>RTFLNLTKPLCEVNSWHILSKDNAIRIGEDAHILVTREPYLSCDPQGCRMFALSQGTTLRGRHANGTIHDRSPFRALISWEMGQAPSPYNTRVECIGWSSTSCHDGMSRMSICMSGPNNNASAVVWYGGRPITEIPSWAGNILRTQESECVCHKGVCPVVMTDGPANNRAATKIIYFKEGKIQKIEELAGNAQHIEECSCYGAGGVIKCICRDNWKGANRPVITIDPEMMTHTSKYLCSKVLTDTSRPNDPTNGNCDAPITGGSPDPGVKGFAFLDGENSWLGRTISK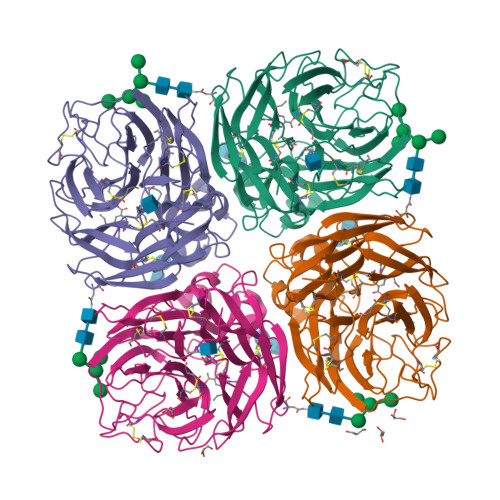DSRSGYEMLKVPNAETDIQSGPISNQVIVNNQNWSGYSGAFIDYWANKECFNPCFYVELIRGRPKESSVLWTSNSIVALCGSKKRLGSWSWHDGAEIIYFE[4x]> MGSQVSTQRSGSHENSNSATEGSTINYT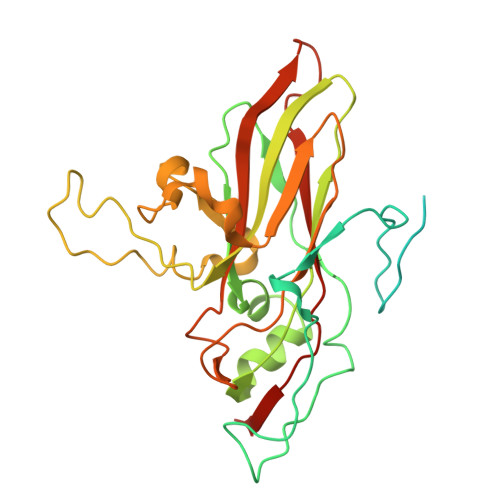TINYYKDSYAATAGKQSLKQDPDKFANPVKDIFTEMAAPLKSPSAEACGYSDRVAQLTIGNSTITTQEAANIIVGYGEWPSYCSDSDATAVDKPTRPDVSVNRFYTLDTKLWEKSSKGWYWKFPDVLTETGVFGQNAQFHYLYRSGFCIHVQCNASKFHQGALLVAILPEYVIGTVAGGTGTEDSHPPYKQTQPGADGFELQHPYVLDAGIPISQLTVCPHQWINLRTNNCATIIVPYINALPFDSALNHCNFGLLVVPISPLDYDQGATPVIPITITLAPMCSEFAGLRQAVTQ> MVRVDVEERFNRIARNTVEIVTEEELKGLLASGARIKGYIGYEPSGVAHIGWLVWMYKVKDLVEAGVDFSVLEATWHAYINDKLGGDMDLIRAAARIVRRVMEAAGVPVERVRFVDAEELASDKDYWGLVIRVAKRASLARVRRALTIMGRRAEEAEVDASKLIYPLMQVSDIFYMDLDIALGGMDQRKAHMLARDVAEKLGRKKPVAIHTPIISSLQGPGRMEASQGEIDDVLAEVKMSKSKPETAVFVVDSDDDIRRKIRKAYCPAKQVQGNPVLEIAR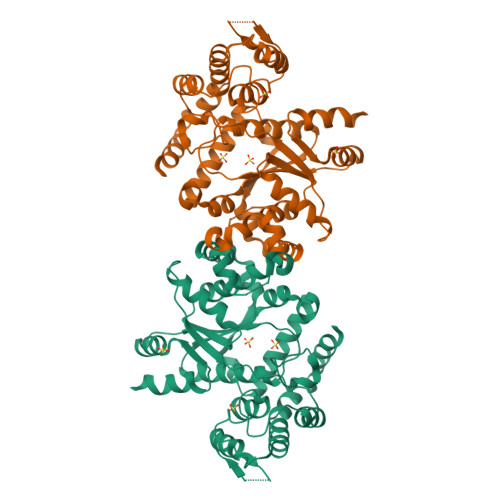YILFARDGFTLRVDRPAKYGGPVEYTSYEELERDYTDGRLHPLDLKNAVAESLIEVVRPIRGAVLGDPAMKRALEAIEGKVTR>IEMKPHPWFFGKIPRAKAEEMLSKQRHDGAFLIRESESAPGDFSLSVKF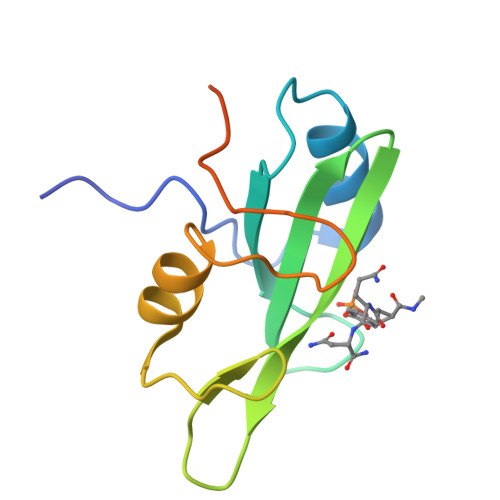GNDVQHFKVLRDGAGKYFLWVVKFNSLNELVDYHRSTSVSRNQQIFLRDIEQVPQQPTYVQAHHHHHH[2x]>SINPKELLDRATTLLEEGDIETAAKVARTAYEHIGENGRHAGAALTLLGQIHVELGDIDAARNYYAAAVKVDEDGSLPEELGGGPEKFLWLAQLSEEGGHDSVAWFERGATVLRAQIQSLMDSLEQRPLSRGQVEAAIADKRRRLAETLCAVVEVYMTDLSWEDDAEQRCEALITEATMIAPEWPETWQTVANVRISQERTEEAREALRRSLGLWTHLPPEDPGVPPFPSRVSLVRLLIEVDMEEEALEVTERLIAEDDLSVEVWYLGGYARYRLGEKEREASGQASEPEAWKDTWRSSRKWLRQCLKVF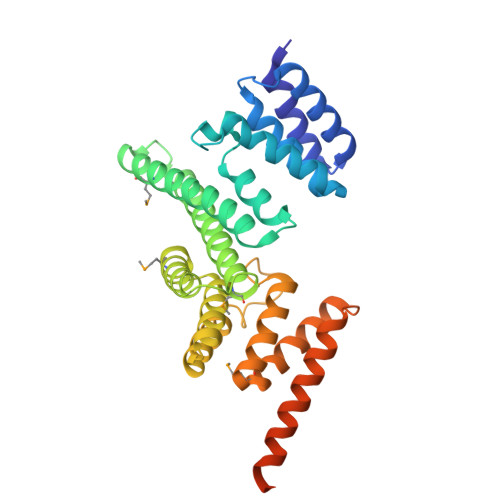EA[2x]> M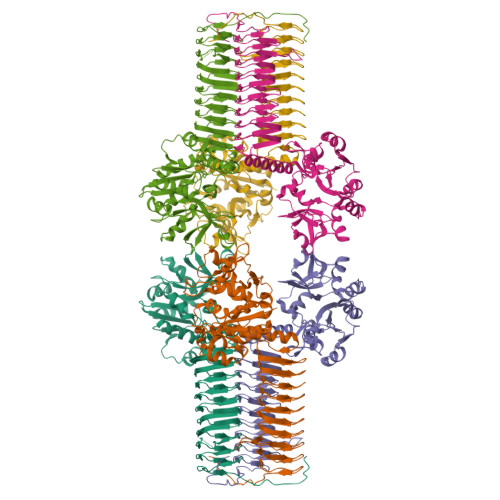SNSSMSVVILAAGKGTRMYSDLPKVLHPLAGKPMVQHVIDAAMKLGAQHVHLVYGHGGELLKKTLADPSLNWVLQAEQLGTGHAMQQAAPHFADDEDILMLYGDVPLISVDTLQRLLAAKPEGGIGLLTVKLDNPSGYGRIVRENGDVVGIVEHKDASDAQREINEINTGILVANGRDLKRWLSLLDNNNAQGEFYITDIIALAHADGKKIATVHPTRLSEVEGVNNRLQLSALERVFQTEQAEKLLLAGVMLLDPSRFDLRGELTHGRDITIDTNVIIEGHVILGDRVRIGTGCVLKNCVIGDDSEISPYTVLEDARLDANCTVGPFARLRPGAELAEGAHVGNFVEIKKARLGKGSKAGHLSYLGDAEIGAGVNIGAGTITCNYDGANKFKTIIGDDVFVGSDTQLVAPVTVANGATIGAGTTVTRDVAENELVISRVKQVHIQGWKRPVKKK MrpH resides at the tip of mannose-resistant Proteus-like (MR/P) fimbriae and is required for MR/P-dependent adherence to surfaces. MrpH is a two-domain adhesin (TDA) consisting of an N-terminal receptor binding domain (NTD) joined through a short linker to a C-terminal pilin domain that attaches the TDA to the fimbrial tip. Although MR/P belongs to a well-known class of adhesive fimbriae encoded by the chaperone-usher pathway, we found that MrpH has a dramatically different structure compared with other tip-located adhesins in this family. Unexpectedly, MrpH was found to bind a zinc cation, which we show is essential for MR/P-mediated biofilm formation and adherence to red blood cells.

The structure of MrpH153 was solved to 1.02 Å resolution using single anomalous dispersion, and the structure of the longer MrpH159 construct solved to 1.75 Å by molecular replacement using MrpH153 as the search model. In both MrpH153 and MrpH159, a metal bound by three histidine (His 72, His 74, His 117) side chains was found. While optimizing crystallization conditions for MrpH153, we carried out thermal shift assay (TSA) experiments to identify conditions that would stabilize the protein and promote crystallization. A melting temperature (Tm) shift from 66.7 ± 0.6°C in 10 mM HEPES buffer, pH 7.5, to 78.5 ± 0.1°C in 10 mM ammonium tartrate pH 7.0, 100 mM NaCl, was observed. Based on the TSA results, ammonium tartrate was added to the MrpH153 protein solution prior to crystallization. Consistent with the significant stabilization of MrpH153 by tartrate in the TSA experiments, a molecule of 1(+)-tartaric acid could be nicely fitted into the electron density for MrpH153, leading to an improved model as indicated by a drop in Rfree of 0.8%-units. One of the tartrate carboxyl oxygens (O1) ligates the Zn2+, completing the tetrahedral co-ordination sphere around the metal, and in addition forms a hydrogen bond to the main chain nitrogen of Arg 118. The second oxygen (O11) from the same carboxyl group forms a hydrogen bond to the main chain nitrogen of Asn 82. Both hydroxyl groups of the tartrate molecule are also involved in hydrogen bond interactions with MrpH153 main chain atoms: O2 with Arg 118 N and the carbonyl oxygen of Thr 116, and O3 with the carbonyl oxygen of Arg 118.

> SIFSYITESTGTPSNATYTYVIERWDPETSGILNPCYGWPVCYVTVNHKHTVNGTGGNPAFQIARIEKLRTLAEVRDVVLKNRSFPIEGQTTHRGPSLNSNQECVGLFYQPNSSGISPRGKLLPGSLCGAHHHHHH>[2x]NTKYNKEFLLYLAGFVDGDGSIIAQIKPNQSYKFKHQL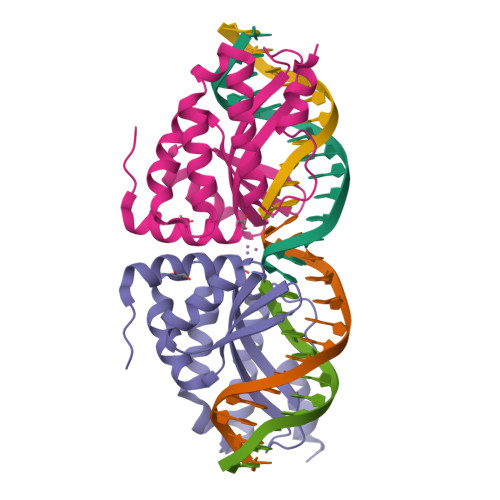SLTFQVTQKTQRRWFLDKLVDEIGVGYVRDRGSVSNYILSEIKPLHNFLTQLQPFLKLKQKQANLVLKIIEQLPSAKESPDKFLEVCTWVDQIAALNDSKTRKTTSETVRAVLDAA>[3x]MLLVGLLSAHNRAVLAQLGCPIKNLDALENAQAIKKKLGKLGRQVLPPSELLDHLFFHYEFQNQRFSAEVLSSLRQLNLAGVRMTPVKCTVVAAVLGSGRHALDEVNLASCQLDPAGLRTLLPVFLRARKLGLQLNSLGPEACKDLRDLLLHDQCQITTLRLSNNPLTAAGVAVLMEGLAGNTSV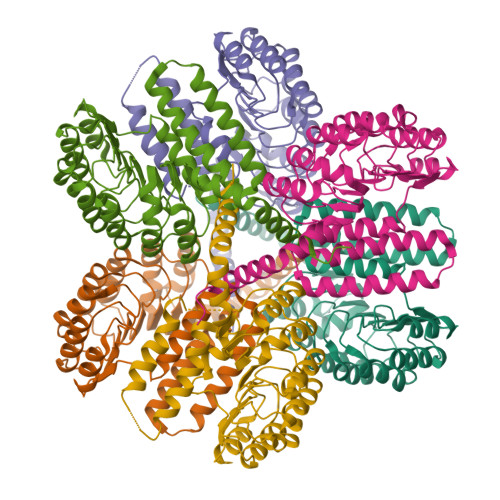THLSLLHTGLGDEGLELLAAQLDRNRQLQELNVAYNGAGDTAALALARAAREHPSLELLHLYFNELSSEGRQVLRDLGGAAEGGARVVVSLTEGTAVSEYWSVILSEVQRNLNSWDRARVQRHLELLLRDLEDSRGATLNPWRKAQLLRVEGEVRALLEQLGSSGSPSGSWSHPQFEKGAGHHHHHH> GPLGSMKLLVVDDSS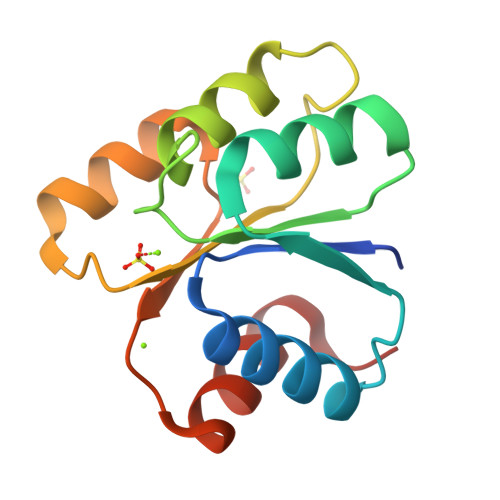TMRRIIKNTLSRLGYEDVLEAEHGVEAWEKLDANADTKVLITDWNMPEMNGLDLVKKVRSDSRFKEIPIIMITAEGGKAEVITALKAGVNNYIVKPFTPQVLKEKLEVVLGTND> MSMSADQVEKLAKNMRKSCLQKIAITEELVDGMRRGEFPDDHDLQCYTTCIMKLLRTFKNGNFDFDMIVKQLEITMPPE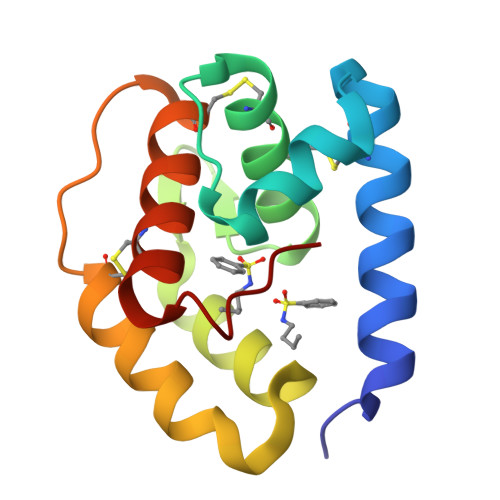EVVIGKEIVAVCRNEEYTGDDCQKTYQYVQCHYKQNPEKFFFP> MAETDGSIPLIPVRMLNEHVYCPRLAYLMWVQGEFSHNEFTVDGVIRHRRVDAGGGVLPSETQEDSRIHARSVSLSSERLGITAKIDLVEGEGAYVSPVDYKRGKRPHVAGGAYEPERVQLCAQGLLLREHGFASDGGALYFVASRERVPVAFDDELIGRTLAAIDEMGRTALSGTMPPPLEDSPKCPRCSLVGICLPDEVRFLSHLSVEPRPIIPADGRGLPLYVQSPKAYVRKDGDCLVIEEERVRVAEARLGETSQVALFGNATLTTAALHECLRREIPVTWLSYGGWFMGHTVSTGHRNVETRTYQYQRSFDPETCLNLARRWIVAKIANCRTLLRRNWRGEGDEAKAPPGLLMSLQDDMRHAMRAPSLEVLLGIEGASAGRYFQHFSRMLRGGDGEGMGFDFTTRNRRPPKDPVNALLSFAYAMLTREWTVALAAVGLDPYRGFYHQPRFGRPALALDMMEPFRPLIADSTVL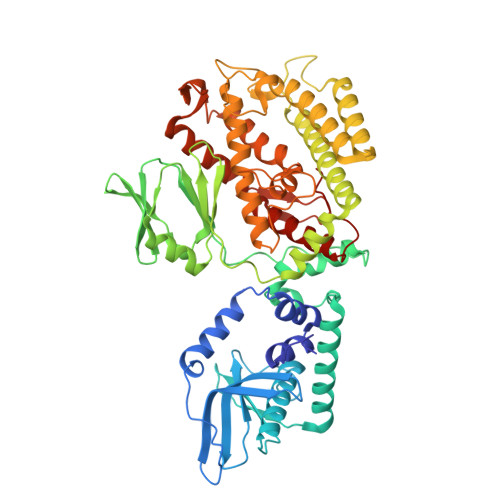MAINNGEIRTGDFVRSAGGCNLTDSARKRFIAGFERRMEQEVTHPIFKYTISYRRLLEVQARLLTRYLSGEIPAYPNFVTR> MAWWKAWIEQEGVTVKSSSHFNPDPDAETLYKAMKGIGTNEQAIIDVLTKRSNTQRQQ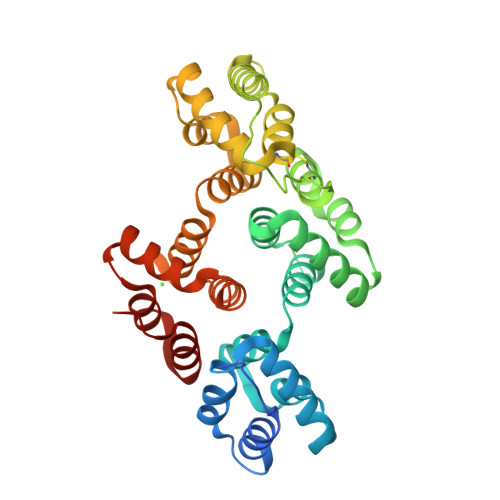IAKSFKAQFGKDLTETLKSELSGKFERLIVALMYPPYRYEAKELHDAMKGLGTKEGVIIEILASRTKNQLREIMKAYEEDYGSSLEEDIQADTSGYLERILVCLLQGSRDDVSSFVDPALALQDAQDLYAAGEKIRGTDEMKFITILCTRSATHLLRVFEEYEKIANKSIEDSIKSETHGSLEEAMLTVVKCTQNLHSYFAERLYYAMKGAGTRDGTLIRNIVSRSEIDLNLIKCHFKKMYGKTLSSMIMEDTSGDYKNALLSLVGSDP5-(3-carboxyphenyl)furan-2-carboxylic 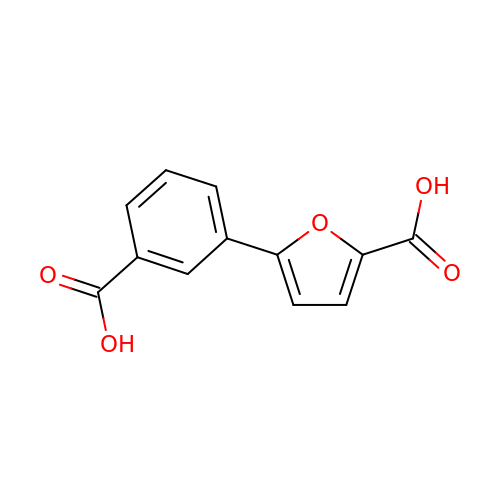acid | C12 H8 O5 | IBQCYMBXLOYXCL-UHFFFAOYSA-N The Streptosporangium sibiricum SibL (Ss-SibL) protein belongs to the S-adenosylmethionine-dependent methyltransferase (SAM-dependent MTase) family. It transfers a methyl group from S-adenosyl-l-methionine (SAM) to 3-hydroxykynurenine (3-HK) to produce S-adenosyl-l-homocysteine (SAH) and 3-hydroxy 4-methyl-kynurenine (3-H4MK). 3-H4MK is the key intermediate needed to synthesize pyrrolo- benzodiazepine (PBD) antitumor antibiotics, including sibiromycin and anthramycin, in Streptomycetes123. Two monomers are tightly intertwined head-to-head, with ~23% total solvent accessible area buried in the dimer interface.

The apo form structure was then solved by molecular replacement. Each ligand-bound subunit of Ss-SibL showed a similar and robust architecture in its peptide backbone, whereas a 2.1 Å r.m.s.d. in the 294 Cα positions was seen in the unbound structure, indicating a considerable conformational rearrangement upon ligand binding. Superposition of apo form and binary complex structures indicates a rotation of the C-terminal domain of approximately 22° toward the N-terminal domain36. A comparison of the unbound and complex structures suggests that SAH binding triggers domain closure to form a pocket favorable for 3-HK binding. When comparing the bound and unbound forms of Ss-SibL we observe that the peptide backbone from strand β6 to helix η5 is shifted by ~4.6 Å to constrict the active site upon substrate binding. In the apo form structure, the nearby acidic residue Asp132 associates directly with Tyr134. Therefore Asp132 can assist the deprotonation. Upon cofactor binding, the shifted Tyr134 is probably ionized and ready for catalysis. The three structures also reveal an open-to-closed conformational change induced by the cofactor, which is required for formation of the substrate-binding site. Based on these observations, a step-wise reaction of SibL can be proposed in which cofactor binding first brings the two domains close together to complete substrate-binding site formation.

>[4x]MSSELSALVPVLFGHAAFQQLNAGCQLGLFELLHERGPLSAEEVADALRLPRRSADILLLGTTALGLSTVTDGGYRNGAPIGAAFRDGLWPVLRDIVQYQDKIAYQPAADYVESLRTGQNAGIRHFPGTTRDLYSRLAAVPGLEELFYRGMHAWSQLSNPVLLAQPDFTRVHRVLDVGGGDAVNAVALARAHPSLRVTVLDRPGALEVARKTIAEAGLEERVRTHAADIFTDSYPAGHDCVLFAHQLVIWSPEQNLTLLRKAYDAVEPGGRVLVFNAFTDDDRTGPLYAALDNVYFTTLPFRHSTIHRWADCESWLREAGFTDVGRTAPPGWTPHGVVSGSRPRAAALEHHHHHH> GPHMGSQYLFLPPN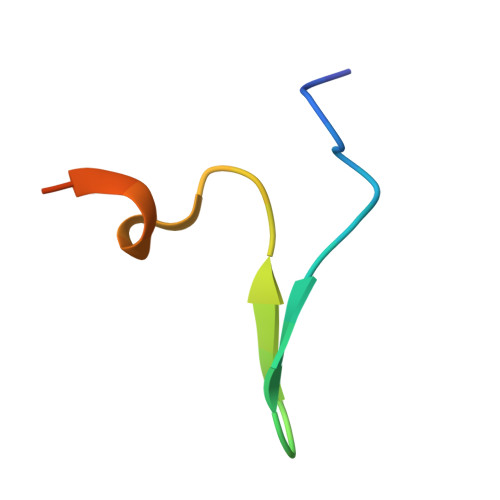RYIFHGAEVYSDSEDDV>[2x]EPSTVIMREAARHGLTIVRLQPQGSRLSLTVQPADFQALMAWLDALGQAGMTTATLAVTAVAQ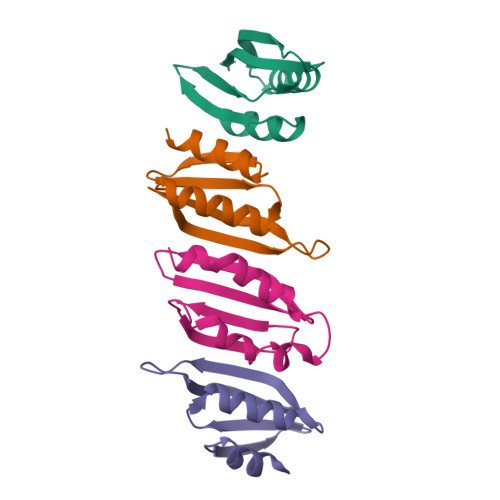QPGWVTVNTLVLER;> TVIMREAARHGLTIVRLQPQGSRLSLTVQPADFQALMAWLDALGQAGMTTATLAVTAVAQQPGWVTVNTLVLER;> PALISRLGALQQIIDDTPGIRLRTLSFDAARNALQLEISAVSSQALEQFSQRARARFRVQTGEMKPRADGIEGRLTLEGA> STLEIAGLVRKNLVQFGVGEKNGSVRWVMNALGVKDDWLLVPSHAYKFEKDYEMMEFYFNRGGTYYSISAGNVVIQSLDVGFQDVVLMKVPTIPKFRDITQHFIKKGDVPRALNRLATLVTTVNGTPMLISEGPLKMEEKATYVHKKNDGTTVDLTVDQAWRGKGEGLPGMCGGAL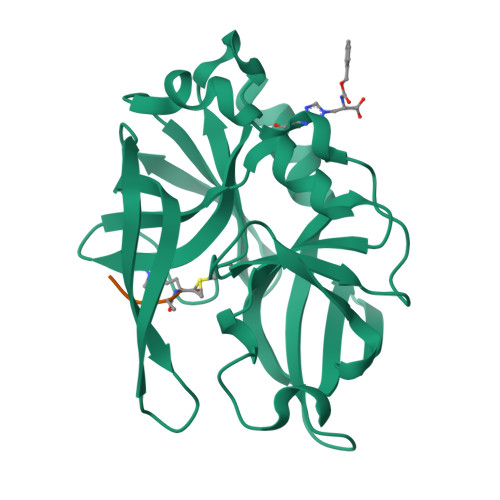VSSNQSIQNAILGIHVAGGNSILVAKLVTQEMFQNI> PTVEE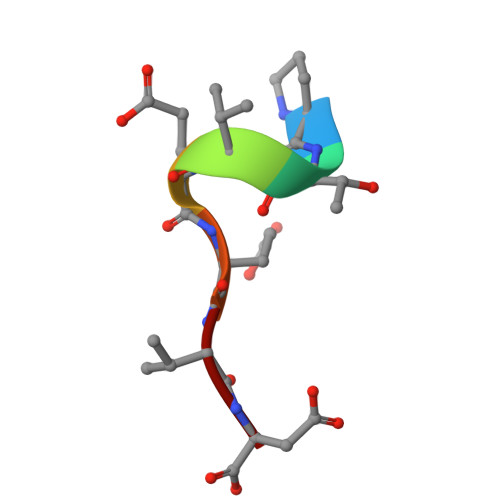VD>[5x]MFVPWQLGTITRHRDELQKLLAASLLPEHPEESLGNPIMTQIHQSLQPSSPCRVCQLLFSLVRDSSTPMGFFEDYACLCFFCLYAPHCWTSTMAAAADLCEIMHLHFPEEEATYGLFGPGRLMGIDLQLHFFVQKCFKTTAAEKILGISNLQFLKSEFIRGMLTGTITCNFCFKTSWPRTDKEEATGPTPCCQITDTTTAPASGIPELARATFCGASRPTKPSLLPALIDIWSTSSELLDEPRPRLIASDMSELKSVVASHDPFFSPPLQADTSQGPCLMHPTLGLRYKNGTASVCLLCECLAAHPEAPKALQTLQCEVMGHIENNVKLVDRIAFVLDNPFAMPYVSDPLLRELIRGCTPQEIHKHLFCDPLCALNAKVVSEDVLFRLPREQEYKKLRASAAAGQLLDANTLFDCEVVQTLVFLFKGLQNARVGKTTSLDIIRELTAQLKRHRLDLAHPSQTSHLYA

In contrast, despite observations that UL32 and its homologs in HCMV (UL52) and KSHV (ORF68) are essential for production of packaged virions, their function in packaging remains unknown. We reveal the structure of KSHV ORF68 and its homolog in EBV (BFLF1), which adopt a novel fold and assemble into homopentameric rings. The central channel of ORF68 is lined with positively charged residues that are necessary for nucleic acid binding and production of infectious virions. We hypothesize that the viral genome is threaded through the ORF68 ring, and that ORF68 acts as a scaffold on which the terminase assembles for genome packaging.

We obtained crystals of ORF68 that diffracted X-rays to a maximum resolution of 2.22 Å and used molecular replacement with the initial cryo-EM model to determine the structure of ORF68. The majority of the protein could be built in the X-ray structure, except for two disordered loops (residues 64–67 and241–262), and a region in the central channel (residues 169–172 and 179–188). ORF68 forms a homopentameric ring with a diameter of ~120 Å. Each monomer contains three zinc fingers and several bundles of α-helices connected by loops. The central channel is constricted toward the top of the ring, with a width of ~25 Å, and widens to ~45 Å at the bottom. Residues 435–451 form an α-helix that is anchored by H452, which coordinates a Zn ion at the bottom of the ring. The subunit interface includes ~1200 Å2 of buried surface area, consisting largely of van der Waals contacts and a stacking interaction between F59 of one subunit and F335 of the adjacent subunit. ORF68 contains several motifs with highly conserved cysteines and histidines. These residues form three CCCH-type zinc fingers, as supported by the tetrahedral coordination geometry, a large anomalous scattering signal, and C/H composition of the putative zinc fingers, along with the previous observation that the homolog from HSV-1, UL32, binds zinc. The third zinc finger (consisting of C191, C192, C415, and H452) is generally conserved in the alpha- and gamma-herpesviruses (with the exception of the closely related model murine gammaherpesvirus MHV68), but is missing in the beta-herpesviruses. This third zinc finger is also atypical in that two coordinating residues, C191 and C192, are adjacent to each other. Mutations K435A (top, more constricted side of the central channel), R443A (middle of the central channel), and K174A/R179A/K182A (henceforth referred to as ‘3+’, in the disordered region of the central channel) all resulted in a drastic reduction in binding affinity, with negligible interactions even at 4 μM ORF68.>[2x]GHHHHHHHHHHSSGHIEGRHMKPSFSPRNYKALSEVQGWKQRMAAKELARQNMDLGFKLLKKLAFYNPGRNIFLSPL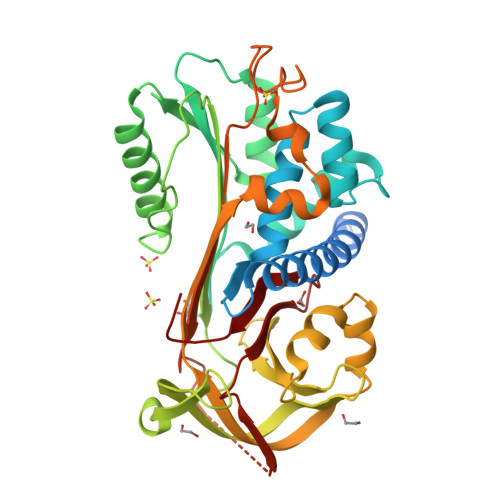SISTAFSMLCLGAQDSTLDEIKQGFNFRKMPEKDLHEGFHYIIHELTQKTQDLKLSIGNTLFIDQRLQPQRKFLEDAKNFYSAETILTNFQNLEMAQKQINDFISQKTHGKINNLIENIDPGTVMLLANYIFFRARWKHEFDPNVTKEEDFFLEKNSSVKVPMMFRSGIYQVGYDDKLSCTILEIPYQKNITAIFILPDEGKLKHLEKGLQVDTFSRWKTLLSRRVVDVSVPRLHMTGTFDLKKTLSYIGVSKIFEEHGDLTKIAPHRSLKVGEAVHKAELKMDERGTEGAAGTGAQTLPMSTPLVVKIDKPYLLLIYSEKIPSVLFLGKIVNPIGK>MGKPFTLSLSSLCLLLLSSACFAISSSKLNECQLNNLNALEPDHRVESEGGLIQTWNSQHPELKCAGVTVSKLTLNRNGLHLPSYSPYPRMIIIAQGKGALGVAIPGCPETFEEPQEQSNRRGSRSQKQQLQDSHQKIRHFNEGDVLVIPPGVPYWTYNTGDEPVVAISLLDTSNFNNQLDQTPRVFYLAGNPDIEYPETMQQQQQQKSHGGRKQGQHQQEEEEEGGSVLSGFSKHFLAQSFNTNEDIAEKLQSPDDERKQIVTVEGGLSVISPKWQEQQDEDEDEDEDDEDEQIPSHPPRRPSHGKREQDEDEDEDEDKPRPSRPSQGKREQDQDQDEDEDEDEDQPRKSREWRSKKTQPRRPRQEEPRERGCETRNGVEENICTLKLHENIARPSRADFYNPKAGRISTLNSLTLPALRQFQLSAQYVVLYKNGIYSPHWNLNANSVIYVTRGQGKVRVVNCQGNAVFDGELRRGQLLVVPQNFVVAEQAGEQGFEYIVFKTHHNAVTSYLKDVFRAIPSEVLAHSYNLRQSQVSELKYEGNWGPLVNPESQQGSPRVKVA[10x]

As the most abundant plant‐derived protein, soy protein isolate (SPI) provides an ideal model for structural studies, with glycinin (11S globulin) and β‐conglycinin (7S globulin) as its major components. Further dissociation of glycinin into its acidic (A) and basic (B) subunits showed that fibrillization was strictly mediated by the acidic subunit (glycinin‐A), which produced well‐defined fibrils, whereas the basic subunit (glycinin‐B) showed no assembly propensity under identical conditions. Removing the Pro164–Ala190 segment resulted in markedly poorer fitting, underscoring the necessity of this region for structural integrity. Together, these structural and computational analyses consistently identify glycinin G4 as the predominant fibril‐forming protein in both polymorphic forms.

PM1 exhibited a characteristic twisted architecture with an 800 Å half‐period twist, corresponding to the 90 nm pitch observed by AFM. To build the atomic model of PM1 and identify the fibril‐constituting protein, we performed de novo model building using ModelAngelo without sequence constraints. Structural analysis further revealed that Val186 resides within the PM1 dimer interface, where spatial constraints favor small residues (e.g., valine in glycinin G4/G5) but exclude bulkier ones (e.g., arginine in glycinin G1/G2/G3). This strongly supports glycinin G4 and G5 as the fibril‐forming proteins. To discriminate between them, we observed that Leu170 in G4 fits the density map more accurately than Pro170 in G5, leading us to select the Pro164‐Ala190 segment of glycinin G4 for final model building. The PM1 core comprises residues Pro164‐Ala190, with Val166‐Leu171, Leu180‐Gln182, and Arg185‐Leu189 forming β‐strands. Importantly, Cryo‐EM analysis of PM1 revealed a structurally unique dual‐core architecture that deviates from conventional amyloid folding patterns. PM1 features spatially segregated hydrophilic (Asp172‐Asn178/Asn178’‐Asp172’) and hydrophobic (Val166‐Ile168/Val186’‐Pro184’) domains, a structural motif distinct from previously characterized amyloid folds in both pathological and functional contexts. The unique dual‐core architecture of PM1 fibrils confers exceptional interfacial properties through precisely organized surface domains. Hydrophobic edge residues (Phe187‐Ala190) facilitate adsorption at oil‐water interfaces, while adjacent hydrophilic regions (Asn177‐Arg185) maintain colloidal stability in aqueous environments.The T5 family of viruses are tailed bacteriophages characterized by a long non-contractile tail. The bacteriophage DT57C is closely related to the paradigmal T5 phage, though it recognizes a different receptor (BtuB) and features highly divergent lateral tail fibers (LTF). We present a composite map determined by electron cryo-microscopy (cryo-EM) at resolutions ranging between 2.9 Å to 4.9 Å of the entire T5-like phage particle DT57C, and atomic models comprising its core structural proteins. Our results provide a complete atomic structure of a T5-like phage, provide insights into the process of DNA ejection as well as a structural basis for the design of engineered phages and future mechanistic studies.

Facilitated by the icosahedral symmetry of the capsid, it was reconstructed at 2.9 Å resolution. Although one of the vertices of the capsid is occupied by the portal complex, icosahedral symmetry was applied to maximize resolution. Consistent with structures of the closely related T5 phage, the T = 13 icosahedral capsid of mature DT57C was composed of two proteins, the major capsid protein (MCP) and the head decorating protein (DCP), and it had a diameter of 930 nm. The asymmetric unit comprises 13 copies of the MCP lacking the Δ-domain (the first 160 N-terminal residues, which is cleaved during the maturation process of the capsid). While one of them is located at an icosahedral vertex and contributes to the formation of pentamers, the remaining 12 form two consecutive proximal and distal hexamers. We observed clear additional map features located at the center of each hexamer, corresponding to the decoration protein. The strongest part of the electron potential map was found at the binding pocket in the center of each hexamer, corresponding to the N-terminal domain. The center of both hexamers, located below the map feature corresponding to the N-terminal domain of DCP, was predicted to be highly negatively charged. Based on the highly negative electrostatic potential at the center of both hexamers, it is likely that the DCP binds to it through such positively charged regions.

>[13x]MTIDINKLKEELGLGDLAKSLEGLTAAQKAQEAERMRKEQEEKELARMNALVSKAVGEDRQKLEQALELVKSLDEKSKKSAELFAQTVEKQQETIVGLQDEIKSLLTAREGRSFVGDSVAKALYGTQETFEDEVEKLVLLSYVMEKGVFETEHGQKHLKAVNQSSSVEVSSESYETIFSQRIIRDLQKELVVGALFEELPMSSKILTMLVEPDAGRATWVAASAYGSDNTTGSEVTGALTEIHFSTYKLAAKSFITDETEEDAIFSLLPLLRKRLIEAHAVSIEEAFMTGDGSGKPKGLLTLASEDSAKVTTEAKADGSVLVTAKTISKLRRKLGRHGLKLSKLVLIVSMDAYYDLLEDEEWQDVAQVGNDAVKLQGQVGRIYGLPVVVSEYFPAKAAGKEFAVIVYKDNFVMPRQRAVTVERERQAGKQRDAYYVTQRVNLQRYFENGVVSGAYAAS> SPNGQTKPLPALKLALEYIVPCMNKHGICVVDDFLGKETGQQIGDEVRALHD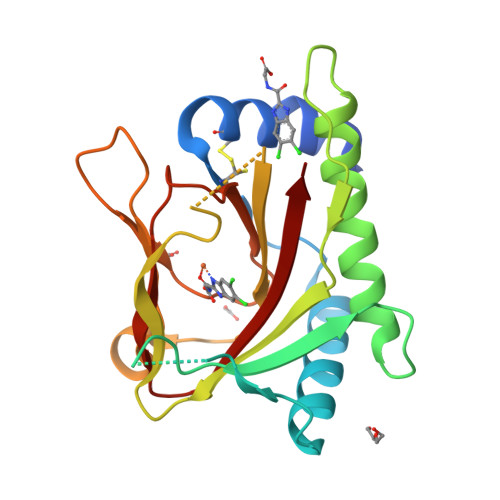TGKFTDGQLVSQKSDSSKDIRGDKITWIEGKEPGCETIGLLMSSMDDLIRHCNGKLGSYKINGRTKAMVACYPGNGTGYVRHVDNPNGDGRCVTCIYYLNKDWDAKVSGGILRIFPEGKAQFADIEPKFDRLLFFWSDRRNPHEVQPAYATRYAITVWYFD>[5x]MGSHHHHHHSQDPMAYSTREILLALCIRDSRVHGNGTLHPV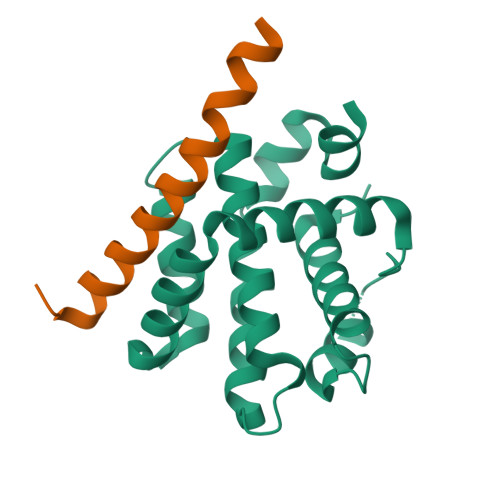LELAARETPLRLSPEDTVVLRYHVLLEEIIERNSETFTETWNRFITHTEHVDLDFNSVFLEIFHRGDPSLGRALAWMAWCMHACRTLCCNQSTPYYVVDLSVRGMLEASEGLDGWIHQQGGWSTLIEDNIPG;>SESQEDIIRNIARHLAQVGDSMDRSIPPGLVNGL[5x]> SMGIINQVSTVTKVIHHELEVAASADDIWTVYSWPGLAKHLPDLLPGAFEKLEIIGDGGVGTILDMTFVPGEFPHEYKEKFILVDNEHRLKKVQMIEGGYLDLGVTYYMDTIHVVPTGKDSCV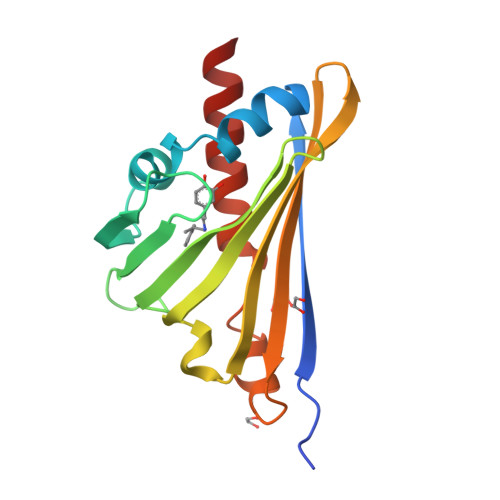IKSSTEYHVKPEFVKIVEPLITTGPLAAMADAISKLVLEHKS>MTVRVAINGFGRIGRNVVRALYESGRRAEITVVAINELADAAGMAHLLKYDTSHGRFAWEVRQERDQLFVGD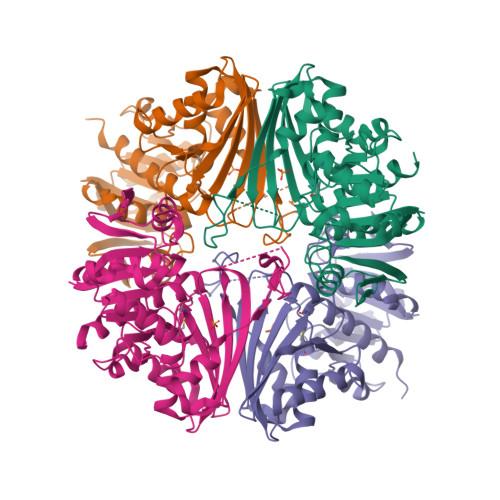DAIRVLHERSLQSLPWRELGVDVVLDCTGVYGSREHGEAHIAAGAKKVLFSHPGSNDLDATVVYGVNQDQLRAEHRIVSNASCTTNCIIPVIKLLDDAYGIESGTVTTIHSAMHDQQVIDAYHPDLRRTRAASQSIIPVDTKLAAGITRFFPQFNDRFEAIAVRVPTINVTAIDLSVTVKKPVKANEVNLLLQKAAQGAFHGIVDYTELPLVSVDFNHDPHSAIVDGTQTRVSGAHLIKTLVWCDNEWGFANRMLDTTLAMATVAFR[4x]> GFVAHVESTCVLNDAGTPQDFTYCVSFNKDLLACWDPDVGKIVPCEFGVLSRLAEIISNILNEQESLIHRLQNGLQDCATHTQPFWDVLTHRTRAPSVRVAQTTPFNTREPVMLACYVWGFYPADVTITWMKNGQLVPSHSNKEKTAQPNGDWTYQTVSYLALTPSYGDVYTCVVQHSG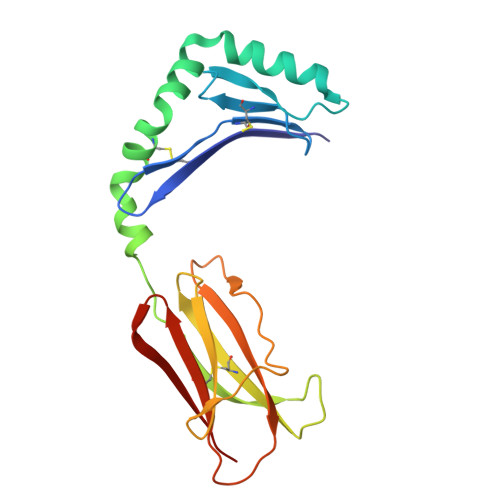TSEPIRGDWTPG>[2x]C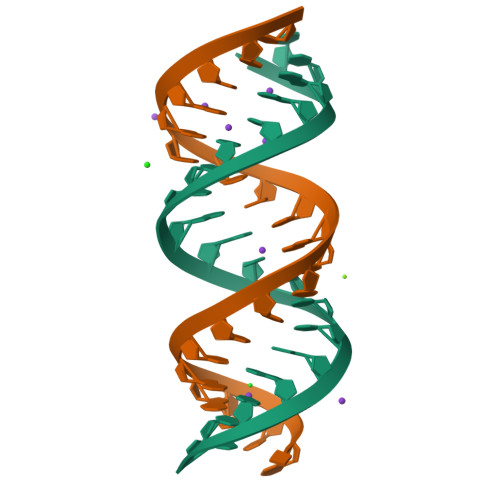CCCGGCCCCGGCCCCGGCCCC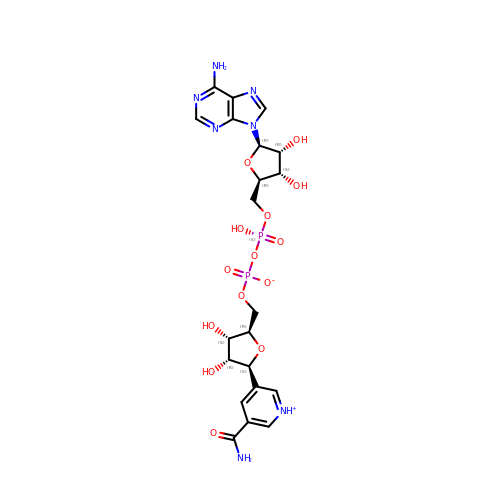5-BETA-D-RIBOFURANOSYLNICOTINAMIDE ADENINE DINUCLEOTIDE | C21 H27 N7 O14 P2 | UINNILASBHZOTM-KMXXXSRASA-N>[12x]MREESWEDHDTIQLTAQRKYLAEVQALETLLTRELSVFLTEPGSKKTNIINRITGKTYALPSTELLRLYEHLEQCRKQGALMYFLERQGTYSGLMLDYDLKLNTNAVPPLEPPALSRLCHRIFVHIKNSSVLPEGSHKIHFFFTLKPEVVQGKYGFHVLIPGLKLAASTKKSIIGSLQHDATVQKILHEQGVTNPESCLDPH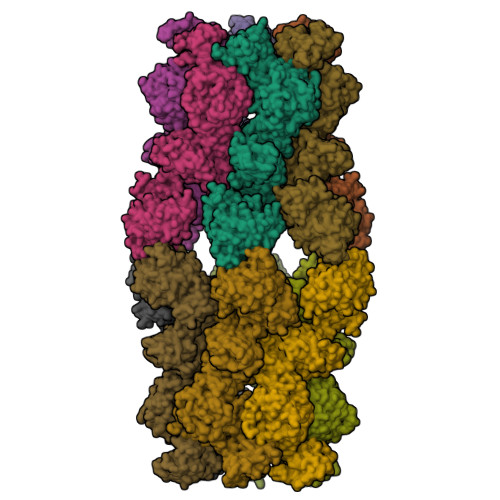SASVPSLLYGSSKLNHKPYQLKTGFELVFDSSDPDYIPIHQIKNLESYNLVSELSLTNEQGSLVRPVYCAADIAAEKEEEIPTEDHSLSILMLHDPEARYLHKILNLLPPEYYVEYPLWSNVVFALANTSANYRPLAEWFSQKCPEKWNTGGKEKLEKLWNDASHHTEKKITKRSIMYWAHKHAPQQYKEIVEQGYFSILAEYVYSYNGMLEHYMIAKVIYAMMGNKFVVDVDSNGKYVWFEFVLPGQPMNQGEIWKWRKEVNPDELHIYISENFSRVMDRITEHIKYHLSQPHESNILNYYKKLLKAFERSKSKIFNDSFKKGVIRQAEFLFRQRSFIQTLDTNPHLLGVGNGVLSIETIPAKLINHFHEHPIHQYTHICYVPFNPENPWTKLLLNALQDIIPELDARLWIMFYLSTAIFRGLKEALMLLWLGGGCNGKTFLMRLVAMVLGDHYASKLNISLLTSCRETAEKPNSAFMRLKGRGYGYFEETNKSEVLNTSRLKEMVNPGDVTARELNQKQESFQMTATMVAASNYNFIIDTTDHGTWRRLRHYRSKVKFCHNPDPSNPYEKKEDPRFIHEYIMDPDCQNAFFSILVYFWEKLQKEYNGQIKKVFCPTIESETEAYRKSQDTLHRFITERVVESPSAETVYNLSEVVTAYAEWYNTNINVKRHIALELSQELENSVLEKYLQWSPNKTRILKGCRILHKFETLQPGESYIGVSTAGTLLNTPICEPKNKWWEWSPNPSAPPEKEASAPTP> TIMPXDI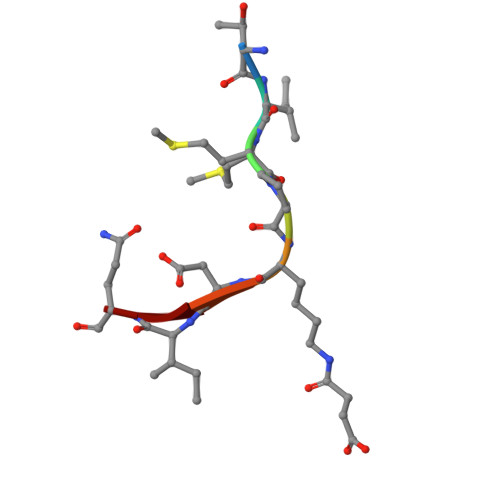Q> LLPTLPKLP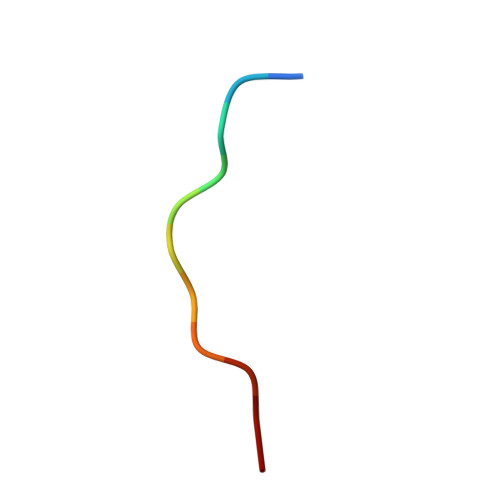SL>[2x]MTASAPDGRPGQPEATNRRSQLKSDRRFQLLAAAERLFAERGFLAVRLEDIGAAAGVSGPAIYRHFPNKESLLVELLVGVSARLLAGARDVTTRSANLAAALDGLIEFHLDFALGEADLI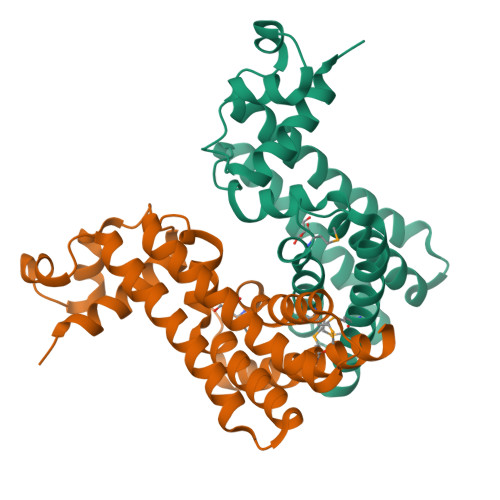RIQDRDLAHLPAVAERQVRKAQRQYVEVWVGVLRELNPGLAEADARLMAHAVFGLLNSTPHSMKAADSKPARTVRARAVLRAMTVAALSAADRCL> GSHMWGFQDSDGDSQPFSLQETYEAKRKEFLSELQRKEEEMRQMFVNKVKETELELKEKERELHEKF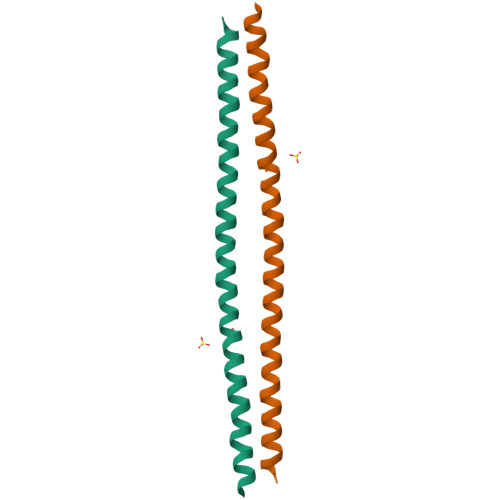EHLKRVHQEEKRKVEEKRRELEEETNAFNRRKAAVEALQSQALHATSQQPLRKDKDKKN>[2x]MGKERKLHNEVLGILGRVGEGNLPKMK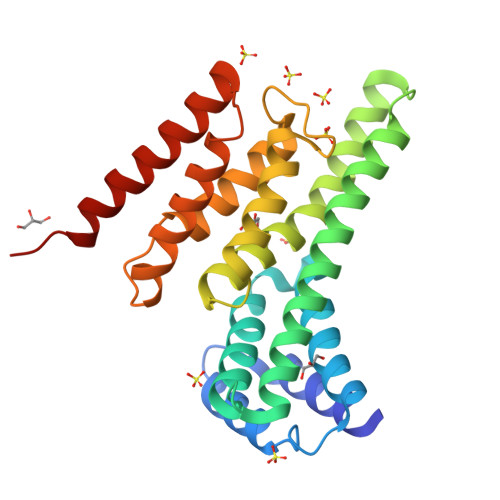EELTNLPIRQSTDKEIQDVIQVIFNKSIQPEDSIFVPYYVKLVVSLINDIGEGEPAGRFIRNAIIRQCQRTFENAEEAQAQLEREIANLPEEEAEQRRLIFAGKQKANINFLGLLFTHGLVREKVVLHVLEWLLYGTERKRRFPADYELIHFMNLLLTCGKSFSKEGQEFVPKFRAVLEELMHMHPQRRMQFLLLNTVETIDNNWILEHHHHHH4-[[4-[(6-CHLORO-2-NAPHTHALENYL)SULFONYL]-6-OXO-1-[[1-(4-PYRIDINYL)-4-PIPERIDINYL]METHYL]-2-PIPERAZINYL]CARBONYL]MORPHOLINE | C30 H34 Cl 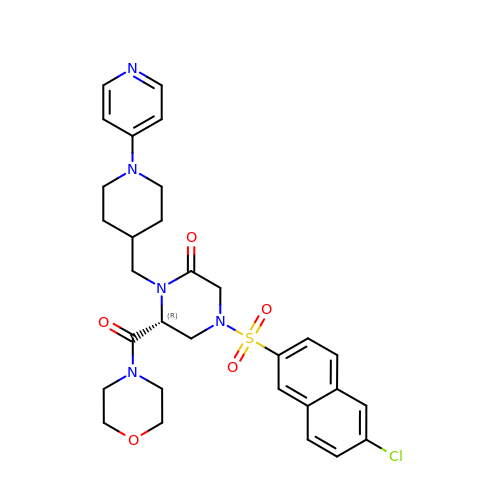N5 O5 S | CJERKHNRUGRCIY-MUUNZHRXSA-N>[5x]MNSYVKEIPDVLQSQYGINCLTDICHYSFNEFRQQVSDHLSWSETNRLYRDAQQEQKENQLYEARILKRANPQLQNAVHLGITLPHAELRGYNSEFGGRASQYVAPGSVSSMFSPAAYLTELYREARNLHASDSVYHLDERRPDLQSMTLSQQNMDTELSTLSLSNEILLKGIKANQSNLDSDTKVMEMLSTFRPSGTIPYHDAYENVRKAIQLQDPKLEQFQKSPAVAGLMHQASLLGINNSISPELFNILTEEITEANAEAIYKQNFGDIDPACLAMPEYLKSYYNFSDEELSQFIRKYPDNELNTQKIHLLKINKIILLSQAVNLPFLKLDEIIPEQNITPTVLGKIFLVKYYMQKYNIGTETALILCNDSISQYSYSNQPSQFDRLFNTSPLNGQYFVIEDTNIDLSLNSTDNWHKAVLKRAFNVDDISLYRLLHIANHNNTDGKIANNIKNLSNLYMTKLLADIHQLTIDELYLLLITIGEDKINLYDIDDKELEKLINRLDTLSNWLHTQKWSIYQLFLMTTTNYDKTLTPEIQNLLDTVYNGLQNFDKNKTKLLAAIAPYIAATLQLPSENVAHSILLWADKIKPSENKITAEKFWIWLQNRDTTELSKPPEMQEQIIQYCHCLAQLTMIYRSSGINENAFRLFIEKPTIFGIPDEPNKATPAHNAPTLIILTRFANWVNSLGEKASPILTAFENKTLTAEKLANAMNLDANLLEQASIQAQNYKQVTKENTFSNWQSIDIILQWTNIASNLNISPQGISPLIALDYIKPAQKTPTYAQWENAAIALTAGLDTQQTHTLHVFLDESRSTALSNYYIGKVANRAASIKSRDDLYQYLLIDNQVSAEIKTTRIAEAIASIQLYVNRALENIEIHAVSDVITRQFFIDWDKYNKRYSTWAGVSQLVYYPENYIDPTMRIGQTKMMDTLLQSVSQSQLNADTVEDAFKSYLTSFEQVANLEVISAYHDNVNNDQGLTYFIGNSKTEVNQYYWRSVDHSKFNDGKFAANAWSEWHKIDCAINPYQSTIRPVIYKSRLYLIWLEQKETAKQKEDNKVTTDYHYELKLAHIRYDGTWNVPITFDVDEKILALELTKSQAPGLYCAGYQGEDTLLIMFYRKKEKLDDYKTAPMQGFYIFSDMSSKDMTNEQCNSYRDNGYTHFDTNSDTNSVIRINNRYAEDYEIPSLINHSNSHDWGEYNLSQVYGGNIVINYKVTSNDLKIYISPKLRIIHDGKEGRERIQSNLIKKYGKLGDKFIIYTSLGINPNNSSNRFMFYPVYQYNGNTSGLAQGRLLFHRDTSYSSKVAAWIPGAGRSLINENANIGDDCAEDSVNKPDDLKQYIYMTDSKGTATDVSGPVDINTAISSEKVQITIKAGKEYSLTANKDVSVQPSPSFEEMCYQFNALEIDGSNLNFTNNSASIDVTFTALADDGRKLGYEIFNIPVIQKVKTDNALTLFHDENGAQYMQWGAYRIRLNTLFARQLVERANTGIDTILSMETQNIQEPMMGIGAYIELILDKYNPDIHGTNKSFKIIYGDIFKAGDHFPIYQGALSDITQTTVKLFLPRVDNAYGNKNNLYVYAAYQKVETNFIRFVKEDNNKPATFDTTYKNGTFPGLASARVIQTVSEPMDFSGANSLYFWELFYYTPMMVAQRLLHEQNFDEANRWLKYVWSPSGYIVRGQIKNYHWNVRPLLENTSWNSDPLDSVDPDAVAQHDPMHYKVATFMRTLDLLMARGDHAYRQLERDTLNEAKMWYMQALHLLGNKPYLPLSSVWNDPRLDNAAATTTQKAHAYAITSLRQGTQTPALLLRSANTLTDLFLPQINDVMLSYWNKLELRLYNLRHNLSIDGQPLHLPIYATPADPKALLSAAVATSQGGGKLPESFISLWRFPHMLENARSMVTQLIQFG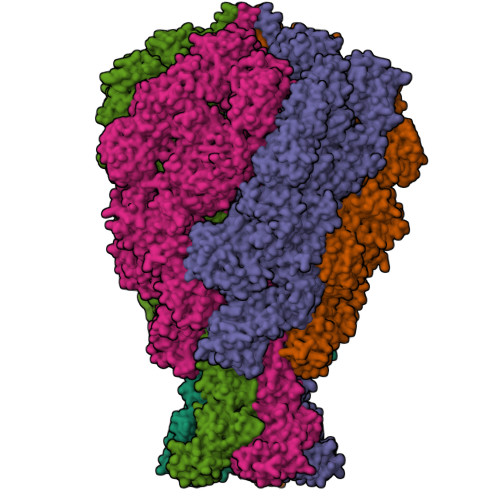STLQNIIERQDAESLNALLQNQAKELILTTLSIQDKTIEEIDAEKTVLEKSKAGAKSRFDNYSKLYDEDVNAGERQALDMRIASQSITSGLKGLHMAAAALEMVPNIYGFAVGGTRYGAIANAIAIGGGIAAEGLLIEAEKVSQSEIWRRRRQEWEIQRNNAEAEMKQIDAQLKSLTVRREAAVLQKTGLKTQQEQTQAQLAFLQRKFSNQALYNWLRGRLAAIYFQFYDLVVARCLMAEQAYRWETNDSSARFIKPGAWQGTYAGLLAGETLMLNLAQMEDAHLKQEQRALEVERTVSLAQVYQSLGEKSFALKDKIEALLQGDKETSAGNDGNQLKLTNNTLSATLTLQDLKLKDDYPEEMQLGKTRRIKQISVSLPALLGPYQDVQAVLSYGGDATGLAKGCKALAVSHGLNDNGQFQLDFNDGKFLPFEGIDINDKGTFTLSFPNAASKQKNILQMLTDIILHIRYTILE3-[4-[2-[3-[[2-[(1~{S})-1-oxidanylethyl]imidazol-1-yl]methyl]-1,2-oxazol-5-yl]ethynyl]phenyl]propan-1-ol 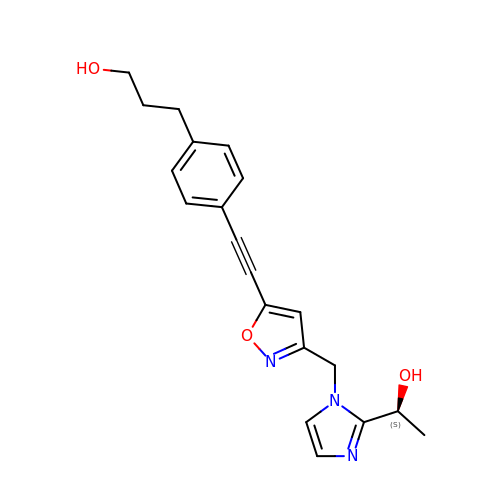| C20 H21 N3 O3 | ADTNNAQOIVHYIK-HNNXBMFYSA-N> MEENKLKFNLQFFADQSDDPDEPGGDGKKGNPDKK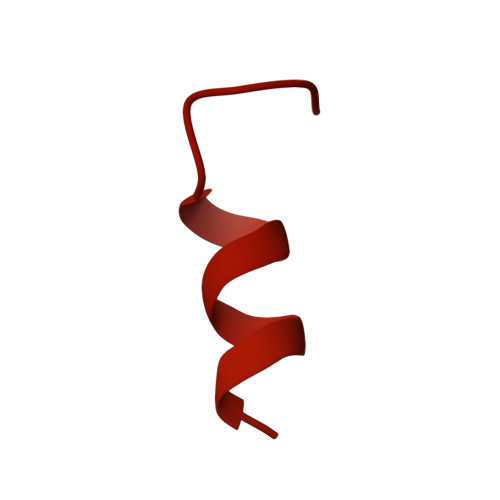ENDEGTEITFTPEQQKKVDEILERRVAHEKKKADEYAKEKAAEAAKEAAKLAKMNKDQKDEYEREQMEKELEQLRSEKQLNEMRSEARKMLSEAEVDSSDEVVNLVVTDTAEQTKSNVEAFSNAVKKAVNEAVKVNARQSPLTGGDSFNHSTKNKPQNLAEIARQKRIIKN> DVSFRLSGADPRSYGMFIKDLRNALPFREKVYNIPLLLPSVSGAGRYLLMHLFNRDGKTITVAVDVTNVYIMGYLADTTSYFFNEPAAELASQYVFRDARRKITLPYSGDYERLQIAAGKPREKIPIGLPALDSAISTLLHYDSTAAAGALLVLIQTTAEAARFKYIEQQIQERAYRDEVPSLATISLENSWSGLSKQIQLAQGNNGIFRTPIVLVDNKGNRVQITNVTSKVVTSNIQLLLNTRNIAEGDNG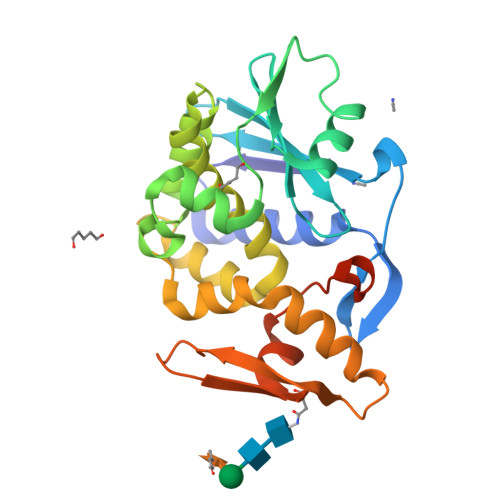DVSTTHGFSSY> MGSSHHHHHHSQDPGWKFSNGKRRPPHKATVTVTDKNGVVKHKS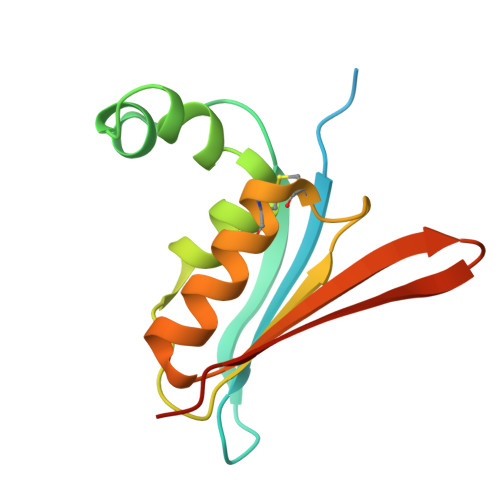NLVSGNMTEAEKKLGFPNNSLATHTENRATRLIDLNQGDTMLIEGQYRPCPRCKGAMRVKAEESGAKVIYTWPEDGDLKKREWEGTPCDKK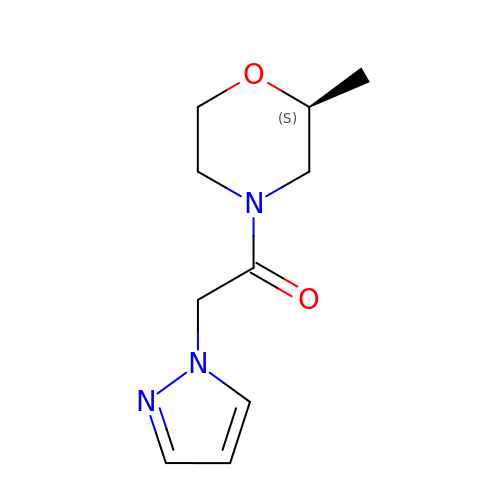1-[(2~{S})-2-methylmorpholin-4-yl]-2-pyrazol-1-yl-ethanone | C10 H15 N3 O2 | YJMLTHJLDUBVIC-VIFPVBQESA-N> GGGRPRWKRHISEQLRRRDRLQRQAFEEIILQYNKLLEKSDLHSVLAQKL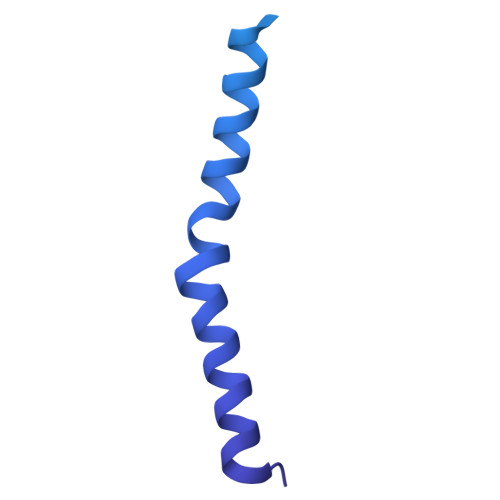QAEKHDVPNRHEISPGHDGTWNDNQLQEMAQLRIKHQEELTELHKKRGELAQLVIDLNNQMQRKDREMQMNEAKIAECLQTISDLETECLDLRTKLCDLERANQTLKDEYDALQITFTALEGKLRKTTEENQELVTRWMAEKAQEANRLNAENEKDSRRRQARLQKELAEAAKEPLPVEQDDDIEVIVDETSDHTEETSPVRAISRAATKRLSQPAGGLLDSITNIFGRRSVSSFPVPQDNVDTHPGSGKE(2R,3S)-2-ethyl-2-[(2E)-2-(6-methoxy-3,4-dihydro-2H-naphthalen-1-ylidene)ethyl]-3-oxidanyl-cyclopentan-1-one 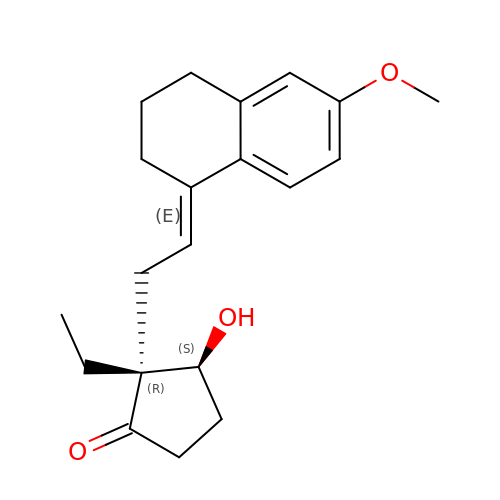| C20 H26 O3 | ZXYHLOFRRMDJAQ-OUBQQWGRSA-N>MANSGCKDVTGPDEESFLYFAYGSNLLTERIHLRNPSAAFFCVARLQDFKLDFGNSQGKTSQTW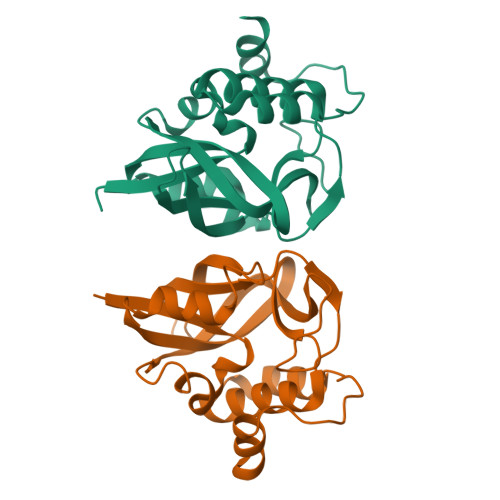HGGIATIFQSPGDEVWGVVWKMNKSNLNSLDEQEGVKSGMYVVIEVKVATQEGKEITCRSYLMTNYESAPPSPQYKKIICMGAKENGLPLEYQEKLKAIEPNDYTGKVSEEIEDIIKKGETQTL[2x]> GAMATDWLGSIVSINCGDSLGVYQGRVSAVDQVSQTISLTRPFHNGVKCLVPEVTFRAGDITELKILEIPGP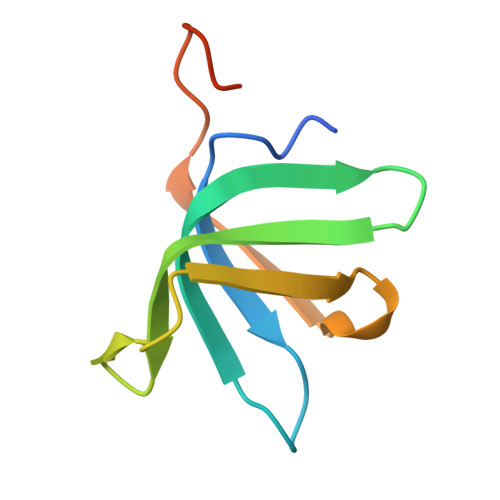GDNQHFGDLHQT>[2x]SNAMNDIVASTQLPNTIKTITNDLRKLGLKKGMTVIVHSSLSSIGWISGGAVAVVEALMEVITEEGTIIMPTQSSDLSDPKHWSRPPVPEEWWQIIRDNVPAFEPHITPTRAMGKVVECFRTYPNVVRSNHPLGSFAAWGRHAEEITVNQSLSMSLGEESPLRKIYDLDGYILLIGVGYDSNTSVHLSEVRSGACELIKVGAPIIENGERV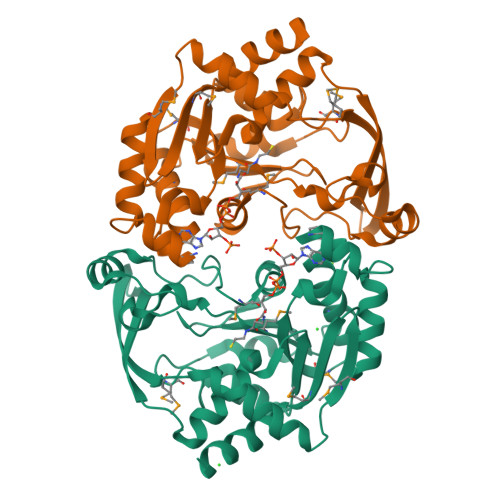WKEFVDMDYDSDKFVEIGVEFEQKGTVTMGKIGNAKCRLMKQRDIVDFGTEWFRKKN2-AMINO-4-[4-(4-AMINO-4-CARBOXY-BUTYRYLAMINO)-5,8,19,22-TETRAOXO-1,2-DITHIA-6,9,13,18,21-PENTAAZA-CYCLOTETRACOS-23-YLCARBAMOYL]-BUTYRIC 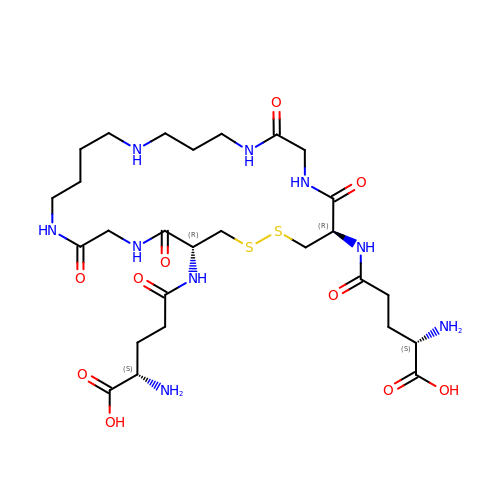ACID | C27 H47 N9 O10 S2 | LZMSXDHGHZKXJD-VJANTYMQSA-N> GDPVEDIIHDALSSTVRRAITSGQDVNTAAGTAPSSHRLETGRVPALQAAETGATSNATDENMIETRCVMNRNGVLEATISHFFSRSGLVGVVNLTDGGTDTTGYAVWDIDIMGFVQLRRKCEMFTYMRFNAEFTFVTTTENGEARPFMLQYMYVPPGAPKPTGRDAFQWQTATNPSVFVKLTDPPAQVSVPFMSPASAYQWFYDGYPTFGQHPETSNTTYGQCPNNMMGTFAVRVVSRVASQLKLQTRVYMKLKHVRAWIPRPIRSQPYLLKNFPNYDSSKITYSARDRASIKQANM;> SPSVEACGYSDRVAQLTVGNSSITTQEAANIVLAYGEWPEYCPDTDATAVDKPTRPDVSVNRFYTLDSKMWQENSTGWYWKFPDVLNKTGVFGQNAQFHYLYRSGFCLHVQCNASKFHQGALLVAVIPEFVLAGRGSNTKPNEAPHPGFNTTFPGTAGASFNDPYVLDSGVPLSQSLIYPHQWINLRTNNCATIIVPYINAVPFDSAINHSNFGLIVVPVSPLKYSSGATTAIPITVTIAPLNSEFGGLRQAVSQ;> GLPTELRPGTNQFLTTEDDTAAPILPGFSPTPSIHIPGEVRSLLELCRVETILEVNNTTDATGLNRLLIPVSAQNKADE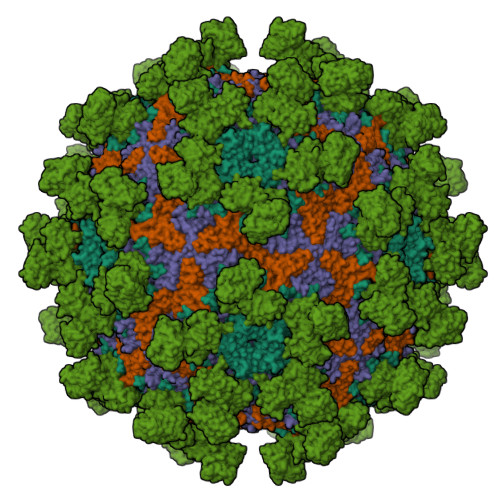LCAAFMVDPGRIGPWQSTLVGQICRYYTQWSGSLKVTFMFTGSFMATGKMLIAYSPPGSAQPANRETAMLGTHVIWDFGLQSSVSLVIPWISNTHFRTAKTGGNYDYYTAGVVTLWYQTNYVVPPETPGEAYIIAMGAAQDNFTLKICKDTDEVTQQAVLQ;> MGAQVSSQRSGSHETGNVATGGSTINFTNINYYKDSYAASASRQDFTQDPKKFTQPVLDSIRELSAPLN;> ETGAPSPGLGPGPECFTANGADYRGTQNWTALQGGKPCLFWNETFQHPYNTLKYPNGEGGLGEHNYCRNPDGDVSPWCYVAEHEDGVYWKYCEIPACQMPGNLGCYKDHGNPPPLTGTSKTSNKLTIQTCISFCRSQRFKFAGMESGYACFCGNNPDYWKYGEAASTECNSVCFGDHTQPCGGDGRIILFDTLVGACGGNYSAMSSVVYSPDFPDTYATGRVCYWTIRVPGASHIHFSFPLFDIRDSADMVELLDGYTHRVLARFHGRSRPPLSFNVSLDFVILYFFSDRINQAQGFAVLYQAVKEEGSENLYFQGGSLPQERPAVNQTVAEVITEQANLSVSAARSSKVLYVITTSPSHPPQTVPGTHHHHHHHHHH> MLEPLRLSQLTVALDARLIGEDAVFSAVSTDSRAIGPGELFIALSGPRFDGHDYLAEVAAKGAVAALVEREVADAPLPQLLVRDTRAALGRLGALNRRKFTGPLAAMTGSSGKTTVKEMLASILRTQAGDAESVLATRGNLNNDLGVPLTLLQLAPQHRSAVIELGASRIGEIAYTVELTRPHVAIITNAGTAHVGEFGGPEKIVEAKGEILEGLAADGTAVLNLDDKAFDTWKARASGRPLLTFSLDRPQADFRAADLQRDARGCMGFRLQGVAGEAQVQLNLLGRHNVANALAAAAAAHALGVPLDGIVAGLQALQPVKGRAVAQLTASGLRVIDDSYNANPASM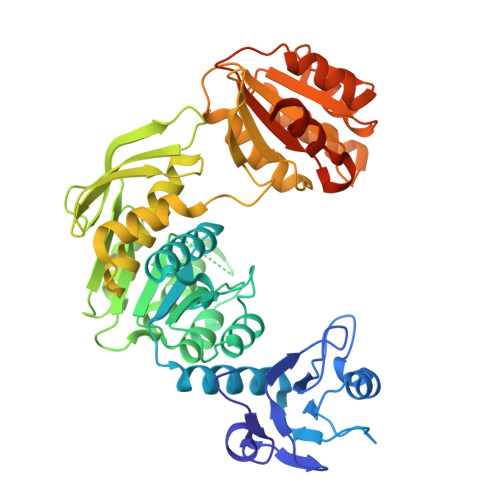LAAIDILSGFSGRTVLVLGDMGELGSWAEQAHREVGAYAAGKVSALYAVGPLMAHAVQAFGATGRHFADQASLIGALATEDPTTTILIKGSRSAAMDKVVAALCGSSEESHSSVDKLAAALEHHHHHH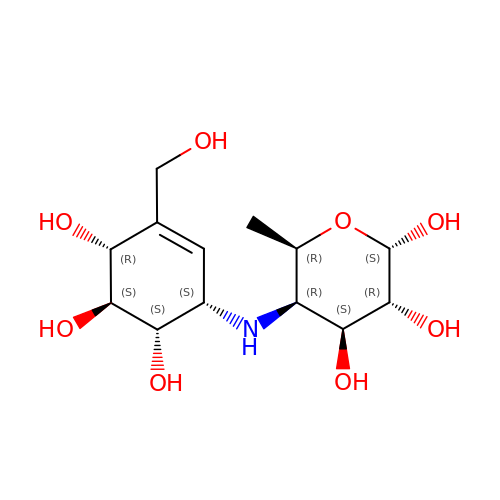(2~{S},3~{R},4~{S},5~{R},6~{R})-5-[[(1~{S},4~{R},5~{S},6~{S})-3-(hydroxymethyl)-4,5,6-tris(oxidanyl)cyclohex-2-en-1-yl]amino]-6-methyl-oxane-2,3,4-triol | C13 H23 N O8 | RBZIIHWPZWOIDU-NLVRWMLHSA-N trans-4-aminocyclohexanol | 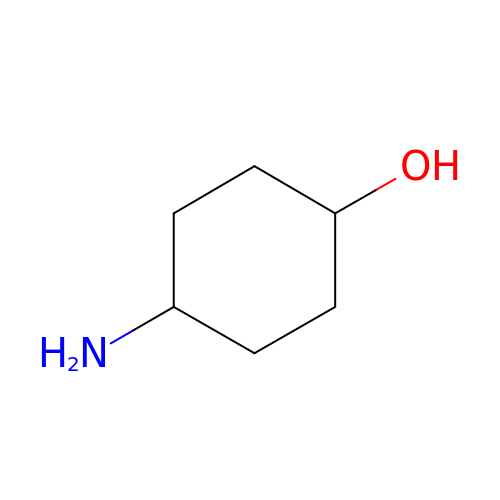C6 H13 N O | IMLXLGZJLAOKJN-IZLXSQMJSA-N> GPLGHMSIFEKDLMAYFDENLNRNWRGREHWKVRNFKKANKSMDTKKKHKQKKVLE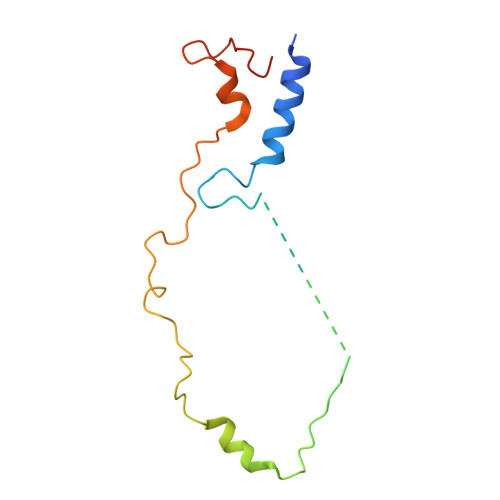IDFFKTDDSFEDKVFASKGRTKIDMPIKNRKNDTHYLLPDDFHFSTDRITRLFIKPGQKMSLFSHRKHT>MIFSVRGEVLEVALDHAVIEAAGIGYRVNATPSALATLRQGSQARLVTAMVVREDSMTLYGFSDAENRDLFLALLSVSGVGPRLAMATLAVHDAAALRQALADSDVASLTRVPGIGKRGAERIVLELRDKVGPVGASGLTVGTAADGNAVRGSVVEALVGLGFAAKQ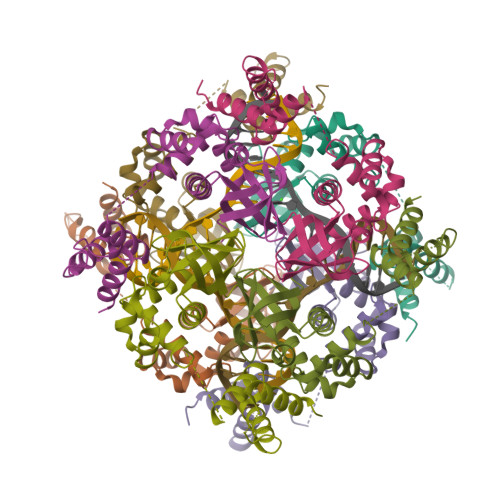AEEATDQVLDGELGKDGAVATSSALRAALSLLGKTR[8x]>MTFTKACSVDEVPPGEALQVSHDAQKVAIFNVDGEFFATQDQCTHGEWSLSEGGYLDGDVVECSLHMGKFCVRTGKVKSPPPCEPLKVYPIRIEGRDVLVDFSRAA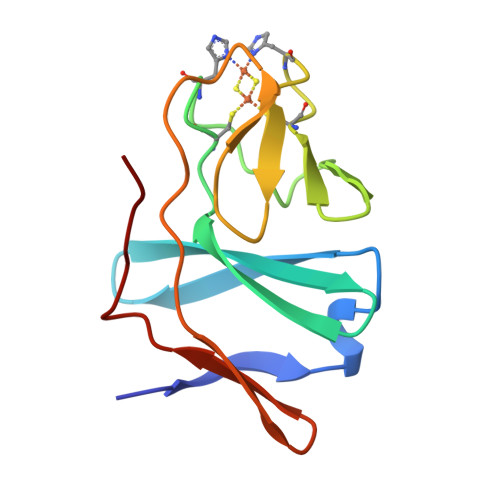LHA[2x]The ubiquitin-proteasome system (UPS) is a crucial regulatory pathway responsible for eliminating damaged or unnecessary proteins within cells. Central to this system is the proteasome, a molecular machine that selectively degrades proteins. A hydrophobic-tyrosine-any residue (HbYX) motif on the C-termini of proteasome-activating complexes independently triggers gate-opening of the 20S core particle for protein degradation; however, the causal allosteric mechanism remains unclear. The architecture of the archaeal 20S proteasome is conserved resembling the eukaryotic 20S, but its α and β rings are homoheptameric rather than heteroheptameric.

The structure of the N-terminal tail in the closed gate conformation has not been well resolved in previously published structures of the T20S proteasome; thus, our high-resolution structures of the WT T20S (2.1 Å), ZYA-T20S (1.9 Å), and T20S-αL81Y (2.3 Å) provide insight to how the gate is stabilized in the close and open states. The WT T20S map does show clear pore-central densities that are expected for the closed gate. In addition, our WT map also resolves the N-termini up to Ala11, which includes 2 additional residues not previously resolved in the closed state. Our cryo-EM structure of the WT T20S now resolves more of the N-termini in the closed state, showing clear density beyond the prior resolved T13 to also show the location of I12 and A11. In this T20S model, the T13 side chain occupies the space between Helices 0 and 2 and I12 is seen binding to a hydrophobic pocket created by the neighboring subunits N-termini comprising A11, I12, and V14. Prior studies suggest the N-termini of the closed state in the T20S are disordered, but our WT structure shows a high degree of order up to residue 11 with residues 1-10 being disordered, though still occupying the central channel. For example, in the closed state, I12 is bound to the neighboring N-termini’s hydrophobic pocket, and T13 is bound under Helix 0; then in the open state I12 binds under Helix 0 and T13 binds near V129/R130 in the other neighboring subunit.

>[14x]MQQGQMAYDRAITVFSPDGRLFQVEYAREAVKKGSTALGMKFANGVLLISDKKVRSRLIEQNSIEKIQLIDDYVAAVTSGLVADARVLVDFARISAQQEKVTYGSLVNIENLVKRVADQMQQYTQYGGVRPYGVSLIFAGIDQIGPRLFDCDPAGTINEYKATAIGSGKDAVVSFLEREYKENLPEKEAVTLGIKALKSSLEEGEELKAPEIASITVGNKYRIYDQEEVKKFL;>[14x]MNQTLETGTTTVGITLKDAVIMATERRVTMENFIMHKNGKKLFQIDTYTGMTIAGLVGDAQVLVRYMKAELELYRLQRRVNMPIEAVATLLSNMLNQVKYMPYMVQLLVGGIDTAPHVFSIDAAGGSVEDIYASTGSGSPFVYGVLESQYSEKMTVDEGVDLVIRAISAAKQRDSASGGMIDVAVITRKDGYVQLPTDQIESRIRKLGLIL>GSHMADKELKFLVVDDFSTMRRIVRNLLKELGFNNVEEAEDGVDALNKLQAGGYGFVISDWDMPNMDGLELLKTIRADGAMSALPVLMVTARAKKENII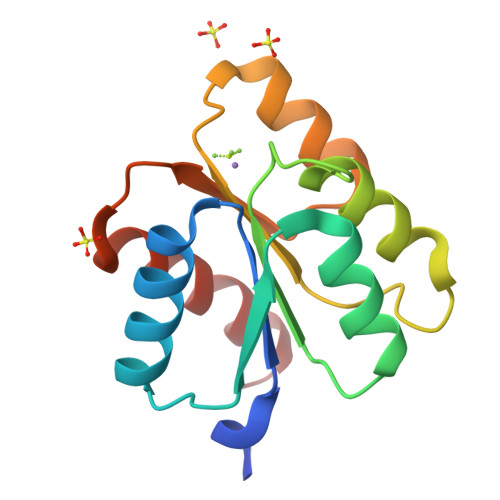AAAQAGASGYVVKPFTAATLEEKLNKIFEKLGM[2x]> LQRLHMLQISYFRDPYHVWYQGNASLGGHLTHVLEGPDTNTTIIQLQPLQEPESWARTQSGLQSYLLQFHGLVRLVHQERTLAFPLTIRCFLGCELPPEGSRAHVFFEVAVNGSSFVSFRPERALWQADTQVTSGVVTFTLQQLNAYNRTRYELREFLEDTCVQYVQ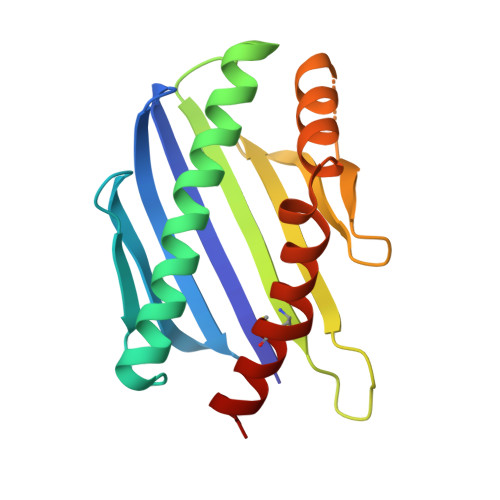KHIS> MQDNSRYTHFLTQRYDAKPQGRDDRYCESIMRRRGLTSPCKDINTFIH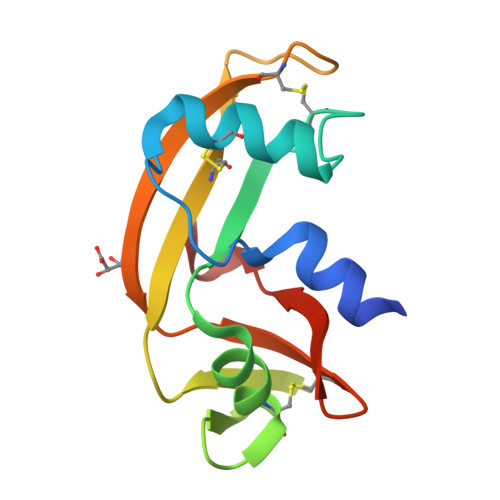GNKRSIKAICENKNGNPHRENLRISKSSFQVTTCKLHGGSPWPPCQYRATAGFRNVVVACENGLPVHLDQSIFRRP> 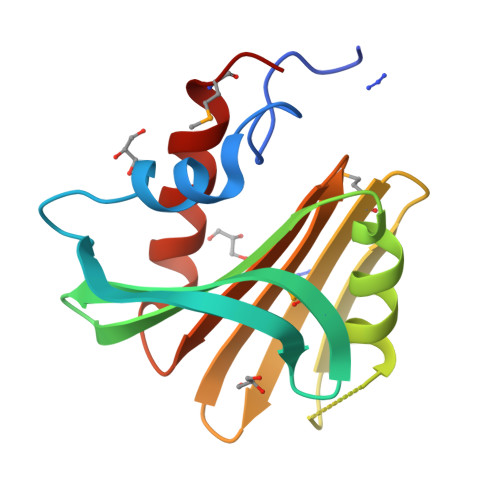MGSDKIHHHHHHPPEAYSLDTAIFVLETRDYRLSDVKEIDSYGDVEMKGKVAVFETEYGPVFLYVYKGEEAKKIWKKLNGRAGFVSIRSVLDLPNMGKFSTVSNGKKIVAWWRKNWLFIVEGKNGVEEFVKHVYRVYEEMKQ> LVHVASVEKGRSYEDFQKVYNAIALKLREDDEYDNYIGYGPVLVRLAWHISGTWDKHDNTGGSYGGTYR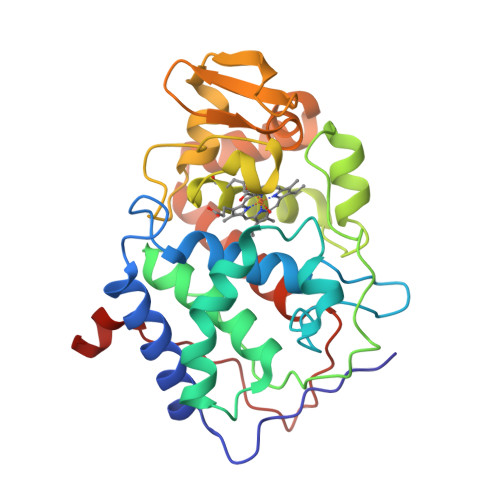FKKEFNDPSNAGLQNGFKFLEPIHKEFPWISSGDLFSLGGVTAVQEMQGPKIPWRCGRVDTPEDTTPDNGRLPDADKDAGYVRTFFQRLNMNDREVVALMGAHALGKTHLKNSGYEGPWGAANNVFTNEYYLNLLNEDWKLEKNDANNEQWDSKSGYMMLPTDYSLIQDPKYLSIVKEYANDQDKFFKDFSKAFEKLLENGITFPKDAPSPFIFKTLEEQGL RIBULOSE-5-PHOSPHATE 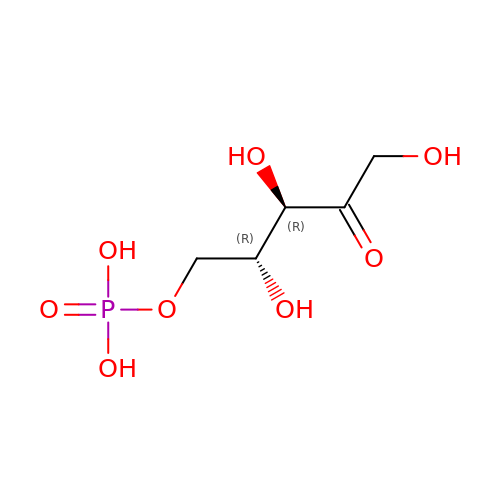| C5 H11 O8 P | FNZLKVNUWIIPSJ-UHNVWZDZSA-N>ASNFTQFVLVDNGGTGDVTVAPSNFANGVAEWISSNSRSQAYKVTCSVRQSSAQNRKYTIKVEVPKVATQTVGGVELPVAAWRSYLNMELTIPIFATNSDCELIVKAMQGLLKDGNPIPSAIAANSGIYANFTQF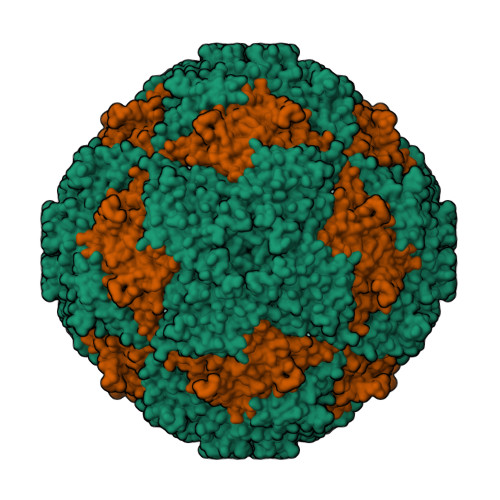VLVDNGGTGDVTVAPSNFANGVAEWISSNSRSQAYKVTCSVRQSSAQNRKYTIKVEVPKVATQTVGGVELPVAAWRSYLNMELTIPIFATNSDCELIVKAMQGLLKDGNPIPSAIAANSGIY[2x]> MELENIV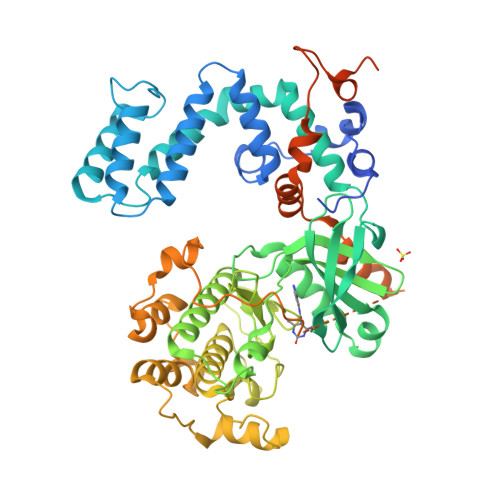ANTVLLKAREGGGGKRKGKSKKWKEILKFPHINQCEDLRRTIDRDYCSLCDKQPVGRLLFRQFCETRPGLESYIQFLDSVAEYEVTPDEKLGEKGKEIMTKYLTPKSPVFITQVGRDLVSQTEEKLLQKPCKELFSACVQSVHDYLRGEPFHEYLDSMYFDRFLQWKWLERQPVTKNTFRQYRVLGKGGFGEVCACQVRATGKMYACKRLEKKRIKKRKGESMALNEKQILEKVNSRFVVNLAYAYETKDALCLVLTIMNGGDLKFHIYNMGNPGFEEERALFYAAEILCGLEDLHHENIVYRDLKPENILLDDYGHIRISDLGLAVKIPEGDLIRGRVGTVGYMAPEVLNNQRYGLSPDYWGLGCLIYEMIEGQSPFRGRKEKVKREEVDRRVLETEEVYSHKFSEEAKSICKMLLTKDAKQRLGCQEEGAAEVKRHPFFRNMNFKRLEAGMLDPPFVPDPRAVYCKDVLDIEQFSTVKGVNLDHTDDDFYSKFSTGSVPIPWQSEMIETECFKELNVFGPHGTLSPDLNRSHPPEPPKKGLLQRLFKRQHQNNSKSSPNSKTSFNHHINSNHVSSNSTGSSVDHHHHHH5-{2-[2-(2,4-dioxo-3,4-dihydropyrimidin-1(2H)-yl)ethoxy]phenoxy}naphthalene-2-carbonitrile | C23 H17 N3 O4 | 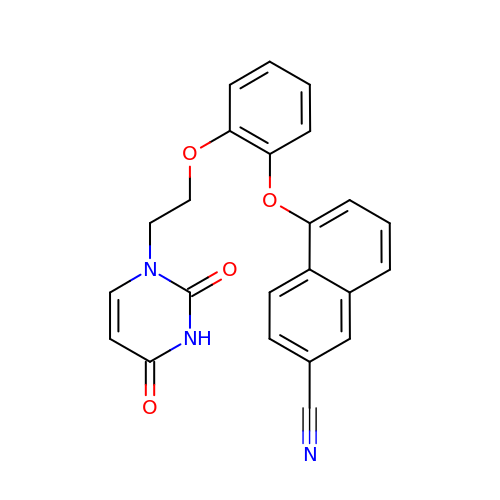OGMGBCQZVDVHAE-UHFFFAOYSA-N>TDTLTRDNGAVVGDNQNSQTAGAQGPVLLQDVQLLQKLQRFDRERIPERVVHARGTGVKGEFTASADISDLSKATVFKSGEKTPVFVRFSSVVHGNHSPETLRDPHGFATKFYTADGNWDLVGNNFPTFFIRDAIKFPDMVHAFKPDPRTNLDNDSRRFDFFSHVPEATRTLTLLYSNEGTPAGYRFMDGNGVHAYKLVNAKGEVHYVKFHWKSLQGIKNLDPKEVAQVQSKDYSHLTNDLVGAIKKGDFPKWDLYVQVLKPEELAKFDFDPLDATKIWPDVPEKKIGQMVLNKNVDNFFQETEQVAMAPANLVPGIEPSEDRLLQGRVFSYADTQMYRLGANGLSLPVNQPKVAVNNGNQDGALNTGHTTSGVNYEPSRLEPRPADDKARYSELPLSGTTQQAKITREQNFKQA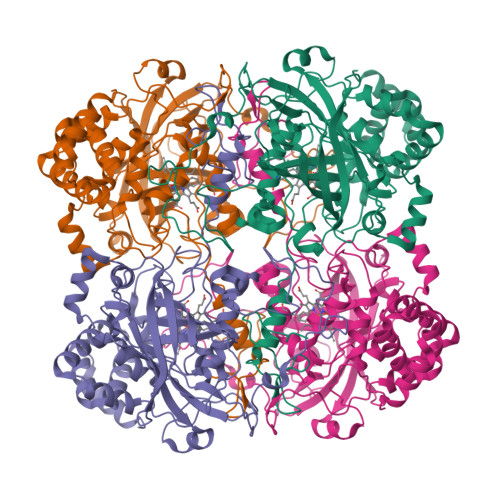GDLYRSYSAKEKTDLVQKFGESLADTLTESKNIMLSYLYKEDPNYGTRVAEVAKGDLSKVKSLAASLKD[4x]>[2x]GVVLYARVSSHDRRSDLDRQVARLTAWATERDLGVGQVVCEVGSGLNGKRPKLRRILSDPDARVIVVEHRDRLARFGVEHLEAALSAQGRRIVVADPGETTDDLVCDMIEVLTGMCARLYGRRGARNRAMRAVTEAKREPGAG

TnpA binds specifically to the transposon ends and is a member of the SR family of DNA exchange enzymes, which are most often associated with site-specific recombination reactions. The SRs found in IS607-family transposable elements, however, are distinguished by the location of their DBDs at their N-termini (experimentally confirmed below). Although there is considerable structural similarity between the catalytic core domains of the subunits, the quaternary structures of the TnpA and smSRs dimers are radically different.

The TnpAISC1926 subunits are shifted apart by about 3 Å relative to TnpAIS1535, the TnpAISC1926 D helices are angled by about 15° rather than being parallel, and the TnpAISC1926 B helices are one turn longer than in TnpAIS1535. The active site serines of each TnpA dimer (TnpAIS1535 residue 59 and TnpAISC1926 residue 74) are separated by 28.6 and 31.5 Å (Cα atoms), respectively. The E helices are interrupted by a four residue β-turn (GRRG in TnpAIS1535 and GMRS in TnpAISC1926) and fold into an antiparallel structure. The split E helices from each subunit associate into a 4-helix bundle, with the C-terminal segments of TnpAIS1535 helix E rotated 35° relative to those of TnpAISC1926. Cysteines were substituted at TnpAIS1535 residues within the catalytic core and helix E region where they would be proximal and oriented appropriately for intersubunit disulfide formation. F126C, located just before the start of helix D, and Q138C at the C-terminal end of helix D efficiently formed dimers after oxidation. Within the helix E bundle, L162C generated substantial amounts of covalently-linked dimers and A182C generated a small amount of dimers after oxidation. These solution results substantiate the dimeric structures observed by crystallography. Nevertheless, we show here that the quaternary structure of the catalytic domain is active for assembling PECs, as evidenced by the robust formation of PECs by IS1535 TnpA dimers covalently crosslinked over the core subunit interface. TnpAIS1535 CTD native and Se-met data were both collected to 2.5 Å resolution, and integrated and scaled using XDS.>MVRSSSRTPSDKPVAHVVANPQAEGQLQWLNRRANALLANGVELRDNQLVVPSEGLYLIYSQVLFKGQGCPSTHVLLTHTISRIAVSYQTKVNLLSAIKSPCQRETPEGAEAKPWYEPIYLGGVFQLEKGDRLSAEINRPDYLDFAESGQVYFG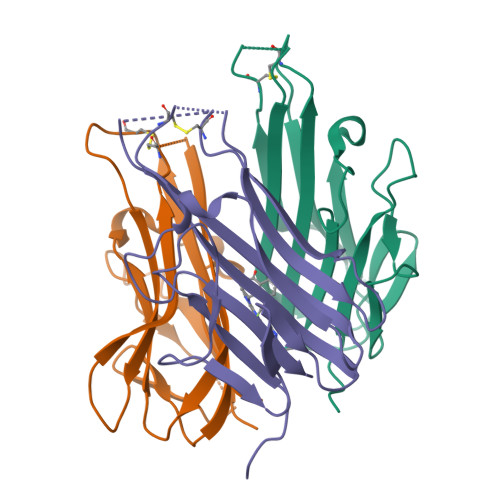IIAL[6x]> MSMLKREDWYDLTRTTNWTPKYVTENELFPEEMSGARGISMEAWEKYDEPYKITYPEYVSIQREKDSGAYSIKAALERDGFVDRADPGWVSTMQLHFGAIALEEYAASTAEARMARFAKAPGNRNMATFGMMDENRHGQIQLYFPYANVKRSRKWDWAHKAIHTNEWAAIAARSFFDDMMMTRDSV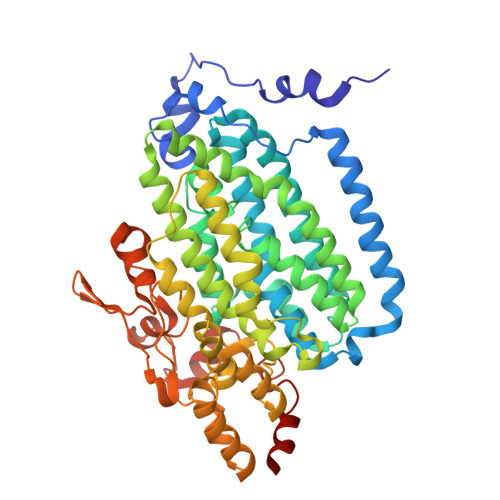AVSIMLTFAFETGFSNMQFLGLAADAAEAGDHTFASLISSIQTDESRHAQQGGPSLKILVENGKKDEAQQMVDVAIWRSWKLFSALTGPIMDYYTPLESRNQSFKEFMLEWIVAQFERQLLDLGLDKPWYWDQFMQDLDETHHGMHLGVWYWRPTVWWDPAAGVSPEEREWLEEKYPGWNDTWGQCWDVITDNLVNGKPELTVPETLPTICNMCNLPIAHTPGNKWNVKDYQLEYEGRLYHFGSEADRWCFQIDPERYKNHTNLVDRFLKGEIQPADLAGALMYMSLEPGVMGDDAHDYEWVKAYQKKTNAA>[2x]MAGARRLELGEALALGSGWRHACHALLYAPDPGMLFGRIPLRYAILMQMRFDGRLGFPGGFVDTQDRSLEDGLNRELREELGEAAAAFRVERTDY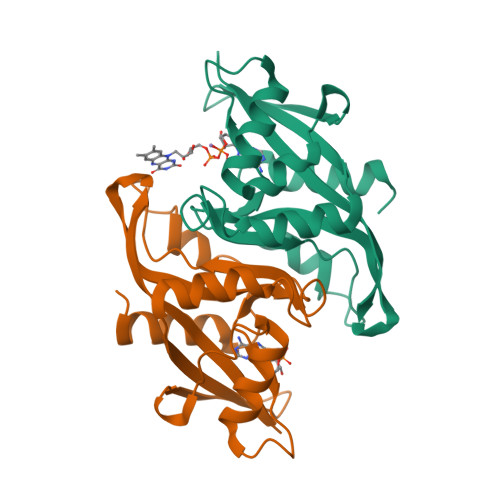RSSHVGSGPRVVAHFYAKRLTLEELLAVEAGATRAKDHGLEVLGLVRVPLYTLRDGVGGLPTFLENSFIGSAREQLLEALQDLGLLQSG> MRVNNGLTPQELEAYGISDVHDIVYNPSYDLLYQEELDPSLTGYERGVLTNLGAVAVDTGIFTGRSPKDKYIVRDDTTRDTFWWADKGKGKNDNKPLSPETWQHLKGLVTRQLSGKRLFVVDAFCGANPDTRLSVRFITEVAWQAHFVKNMFIRPSDEELAGFKPDFIVMNGAKCTNPQWKEQGLNSENFVAFNLTERMQLIGGTWYGGEMKKGMFSMMNYLLPLKGIASMHCSANVGEAGDVAVFFGLSGTGKTTLSTDPARR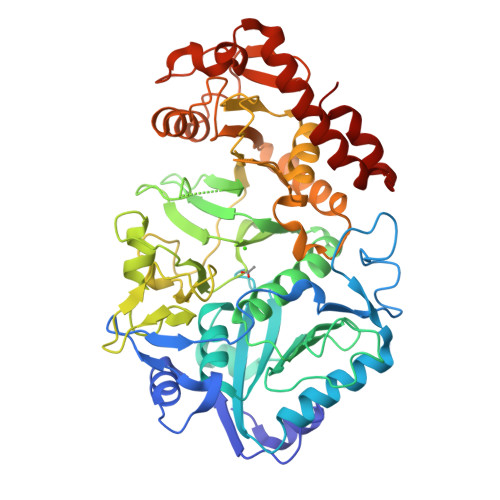LIGDDEHGWDDDGVFNFEGGSYAKTIKLSKEAEPEIYAAIRRDALLENVTKRENGTIDFDDGSKTENTRVSYPIYHIDNIVKPVSKAGHATKVIFLTADAFGVLPPVSRLTADQTQYHFLSGFTAKLAGTERGITEPTPTFSACFGAAFLSLHPTQYAEVLVKRMQAAGAQAYLVNTGWNGTGKRISIKDTRAIIDAILNGSLDNAETFTLPMFNLAIPTELPGVDTGILDPRNTYASPEQWQEKAETLAKLFIDNFDKYTDTPAGAALVAAGPAL> SNAASAAEAPLPQLRAYTVDASWL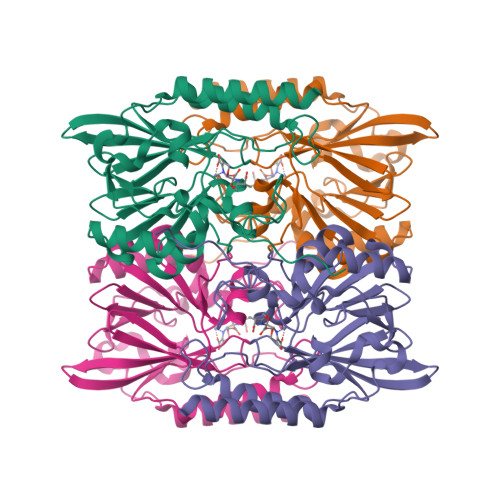QPMAPLQVADHTWQIGTEDLTALLVQTAEGAVLLDGGMPQMAGHLLDNMKLRGVAPQDLRLILLSHAHADHAGPVAELKRRTGAHVAANAETAVLLARGGSNDLHFGDGITYPPASADRIIMDGEVVTVGGIAFTAHFMPGHTPGSTAWTWTDTRDGKPVRIAYADSLSAPGYQLKGNPRYPRLIEDYKRSFATVRALPCDLLLTPHPGASNWNYAVGSKASAEALTCNAYADAAEKKFDAQLARETAGTR> PQMTRENKAPNMSVRAQNVTVSNSRRRRRKNRKPRKQVEQATILKPQLLPGESVAPSGGRGTMDPPVHEICAQSIDPSEGAVGWFYKYMDPAGAVESGKALGEFSKVPDGLLRYSVDAEQRPIVTIECPTVSESDLPLDGKLWRVSFISFPAFRLNFIALANINNEALTLETRNTFIQTLNNITN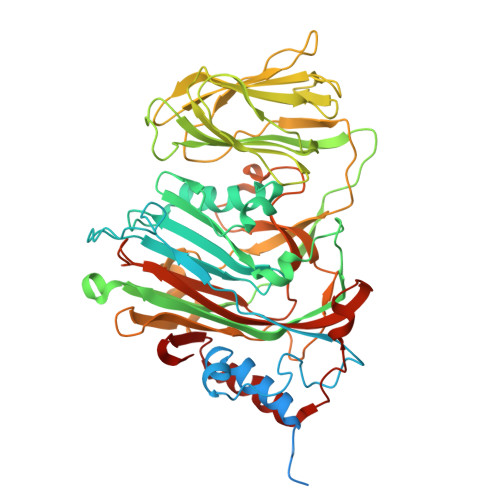WRDLGTGQWAQFAPGWYYSIYVLPNTYAMAEIGDRTDSVTQFRKVYKGITFEFNAPTLIDQGWWVGAHIPVKPQSETIPAAERFSAGSMTVSASNAIFQPSNTVARIVWSITPLPVATVALTTGTGGTNNTSGKFFSVEIDGNVNSVWTFTAPASILAEGEPFAEEGDTTSFSMTTITADTVVYSVSSSLTGSSVIVRGVTKGSGVSITPVTVGIDTEAVNRLSIEMPALTTEEVTTNVPKYEQFLCKESGGAYIVHYKMNNPVFEMTGEENFGGFQFHYPGYDPENNALGLRGIVDTFENNFSSAVVHFWGISQSATIVCKTYDGWEGTTNAGSTVGQFAHTGAEEEDEVVQLANRLQMELTGVYQADDN>MYFDSHLHSEGLGFSELVKLKENGIKEVCSLAFFPVKPKYPQTMIDVFRKLTEFEPLRCEAAGVKMHPAVGIHPRCIPPDYEFVLGYLEEGEWVAFGEIGLELVTDEEIEVLKSQLELAKR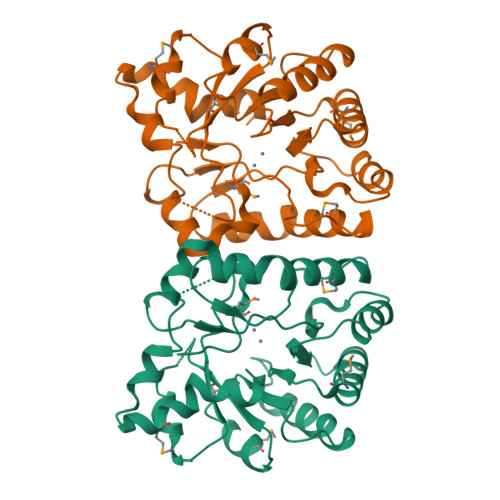MDVPCIIHTPRGNKLKATRKTLEILESLDFPADLAVIDHVNFETLDMVLETEYWIGLTVQPGKLSAEDAARIVAEHGPERFMLNSDAGYRDVEITTVAEAAVKIEEAVGREEMEKVARENARKFLRVLEAAALEHHHHHH[4x]D-arabinaric acid | C5 H8 O7 | 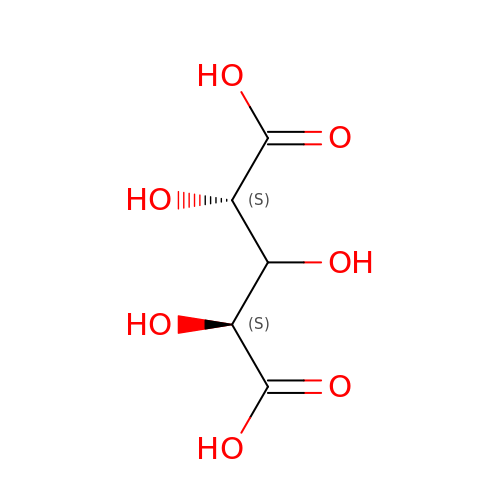NPTTZSYLTYJCPR-HRFVKAFMSA-N>MLKQVEIFTDGSCLGNPGPGGYGAILRYRGREKTFSAGYTRTTNNRMELMAAIVALEALKEHCEVILSTDSQYVRQGITQWIHNWKKRGWKTADKKPVKNVDLWQRLDAALGQHQIKWEWVKGHAGHPENERCDELARAAAMNPTLEDTGYQV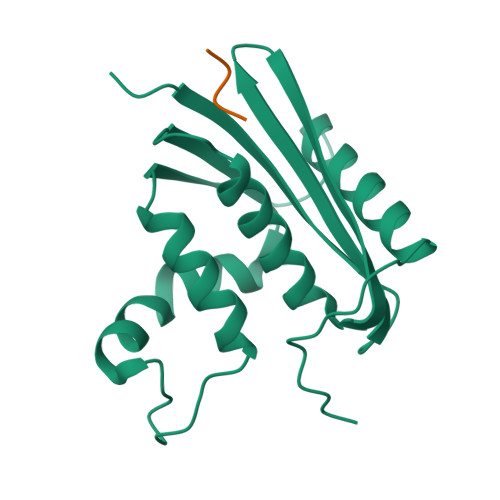EV[2x];>WMDFDDDIPF[2x]3-(4-chloro-1H-pyrrolo[2,3-b]pyridin-2-yl)-5,6-dimethoxy-1-methyl-1H-pyrrolo[3,2-b]pyridine | C17 H15 Cl N4 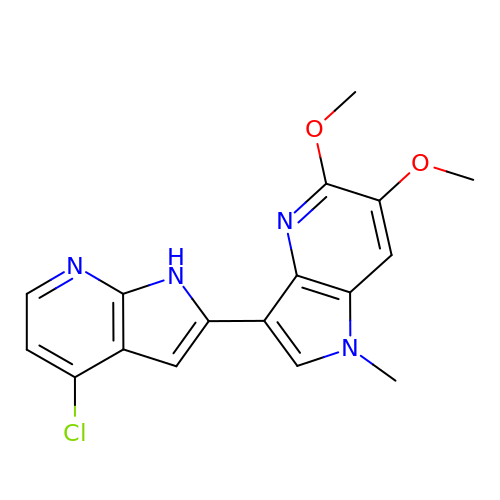O2 | ISLVGFDZMORPFI-UHFFFAOYSA-N> MASASWWKNAVVYQVYPKSFQDSNGDGIGDLQGIISRLDYLEKLGIDAIWLSPVYQSPGVDNGYDISDYEAIDPQYGTMADMDELISKAKEHHIKIVMDLVVNHTSDQHKWFVEAKKGKDNQYRDYYIWRDPVDEHEPNDLKSAFSGSAWKYDERSGQYYLHFFADQQPDLNWQNTELRQKIYNMMNFWLDKGIGGFRMDVIELIGKDPDKNIRENGPMLHPYLQEMNKATFGKRDVMTVGETWNATPKIAEEYSDPDRHELSMVFQFENQSLDQQPGKEKWDLKPLDLGELKKVLVK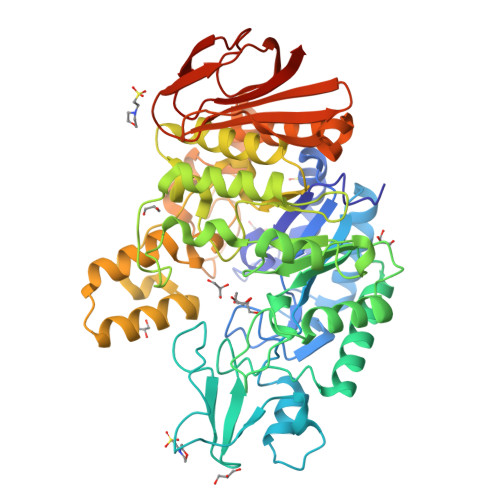WQTKIDFDHAWNSLFWENHDIPRVISRWGNDQEYRVQCAKMFAIILHMMHGTPYIFNGEEIGMTNCPVKNIDEVEDIESINMYNERLAEGYDEEELIHAINVKGRDNARRPMQWNDEKNAGFSEVDPWLSVNPNYKDINVENALADPNSIFYTYQKLIKLRHENPIVVDGDFSLVSNTQDAVLAYYRILNDKKWLVVANLSNEEQNFVSNDQIETILSNYPERNNVQNITLKPYEAFISKVIELEHHHHHH Here, we report structural and functional characteristics of a single-domain AA11 LPMO from Aspergillus fumigatus, AfAA11A. Using a single copper ion cofactor, bound in a highly conserved so-called histidine brace, LPMOs carry out oxidative cleavage of glycosidic bonds using molecular oxygen (O2) or hydrogen peroxide (H2O2) as a cosubstrate. For chitin-active LPMOs, only C1-oxidizing activity has been reported. The catalytic activity of AfAA11A on chitin increases when supplying reactions with hydrogen peroxide, showing that, like LPMOs from other families, AfAA11A has peroxygenase activity. These results show that, in stark contrast to the previously characterized AfAA11B from the same organism, AfAA11A likely plays a role in fungal chitin turnover.

Only one of the conditions tested resulted in a protein crystal suitable for structure analysis, for the de-N-glycosylated protein. The structure of AfAA11A was solved by X-ray crystallography, and a complete structure was obtained, which, however, lacked a bound metal ion in the histidine brace. Of note, except for one GlcNAc attached to Asn62, the structure of this N-deglycosylated protein showed no other signs of N-glycosylation or O-glycosylation. The structure of AfAA11A shows a typical LPMO fold with a core composed of β-strands that are connected by several loops and a few short helices. The core of the protein consists of two β-sheets formed by antiparallel β-strands, which are arranged in an immunoglobulin-like β-sandwich fold. AfAA11A contains a typical LPMO copper-binding site comprised of the nonmethylated N-terminal histidine and His71. The axial copper coordination positions are occupied by the hydroxyl group of Tyr133 and the methyl side chain of Ala69. Relative to AoAA11, AfAA11A has an insertion spanning residues 16 to 26, which contains a surface-exposed tyrosine, Tyr25, in a position similar to that of Tyr27 in CBP21 (SmAA10A), a chitin-active AA10 (38). Because of the Tyr25-containing insertion that is unique for AfAA11A, the substrate-binding surface of this enzyme shows features that are characteristic for chitin-active AA10 LPMOs, such as CBP21, in particular the presence of exposed Tyr25. Interestingly, both AA11 enzymes as well as CBP21 contain a small pocket close to the histidine brace, which has been previously associated with chitin-active LPMOs.

> HMEMSWPYPLRSRFDPQVPEEDIDYSMTSPLNSDGSNFPCKGYQTNTPWRATAQYTAGQTYNMTITGSATHGGGSCQLSLSYDNGKTFKVIQSMEGGCPLVSKYNFKIPGDVANGQALFAWTWYNLIGNRELYMNCADVVISGGTGTPSSFESAYPDLFVANVGNGCSTVEGRETVFANPGDQVIYGGTVTPSSPAFPICH> VTVDDDDDDNDPENRIA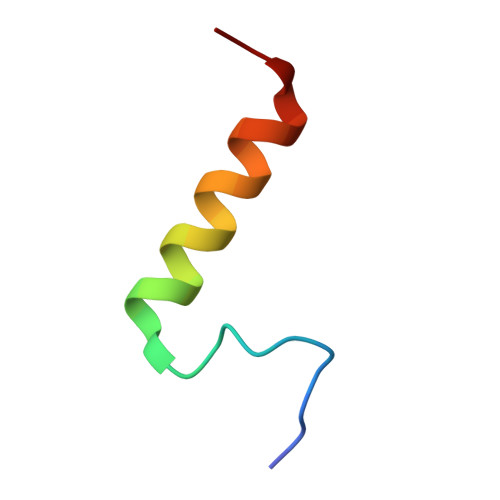KKMLLEEIKANLS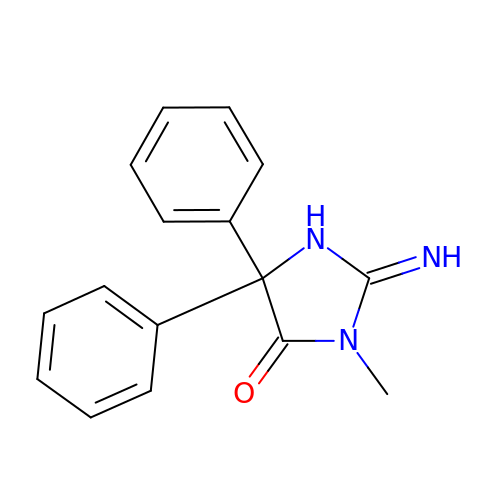(2E)-2-imino-3-methyl-5,5-diphenylimidazolidin-4-one | C16 H15 N3 O | RNWLAFWLSSMCLN-UHFFFAOYSA-N>[6x]MSGPKKYFPIPVEHLEEEIRIRSADDCKQFREEFNSLPSGHIQGTFELANKEENREKNRYPNILPNDHSRVILSQLDGIPCSDYINASYIDGYKEKNKFIAAQGPKQETVNDFWRMVWEQKSATIVMLTNLKERKEEKCHQYWPDQGCWTYGNIRVCVEDCVVLVDYTIRKFCIQPQLPDGCKAPRLVSQLHFTSWPDFGVPFTPIGMLKFLKKVKTLNPVHAGPIVVHCSAGVGRTGTFIVIDAMMAMMHAEQKVDVFEFVSRIRNQRPQMVQTDMQYTFIYQALLEYYLYGDTELDVSSLEKHLQTMHGTTTHFDKIGLEEEFRKLTNVRIMKENMRTGNLPANMKKARVIQIIPYDFNRVILSMKRGQEYTDYINASFIDGYRQKDYFIATQGPLAHTVEDFWRMIWEWKSHTIVMLTEVQEREQDKCYQYWPTEGSVTHGEITIEIKNDTLSEAISIRDFLVTLNQPQARQGEQVRVVRQFHFHGWPEIGIPAEGKGMIDLIAAVQKQQQQTGNHPITVHCSAGAGRTGTFIALSNILERVKAEGLLDVFQAVKSLRLQRPHMVQTLEQYEFCYKVVQDFIDIFSDYAAHHHHHH

Protein tyrosine phosphatases (PTPs) play a critical role in regulating cellular functions by selectively dephosphorylating their substrates. The ∼280 residue PTP catalytic domain consists of an α/β structure, and biochemical and structural studies have led to a detailed understanding of the catalytic mechanism (Barford et al., 1994; Zhang, 2002). Key features of the domain include the PTP signature motif, the mobile Trp-Pro-Asp “WPD” loop that in the closed conformation positions the conserved and catalytically important aspartate residue, and the phosphotyrosine recognition loop. Here we report the crystal structures of 22 PTP domains, including two tandem-domain RPTP structures and a detailed structural comparison of this protein family.

We also report here structures of two tandem-domain RPTPs, RPTPɛ and RPTPγ, revealing the domain organization for the PTP subgroups R4 and R5. Superimposition of all five tandem-domain RPTP structures (CD45, LAR, RPTPσ, RPTPγ, and RPTPɛ) showed that the orientation of the D1 and D2 domains is highly conserved and root mean square deviation (rmsd) values of less than 4.4 Å were obtained, for each pairwise comparison, considering Cα positions of both domains. Surprisingly, sedimentation velocity measurements showed that all single-domain RPTPs studied (IA2, IA2β, GLEPP1, DEP1, and STEP) were entirely monomeric in solution, as were tandem-domain receptor PTPs (RPTPα, CD45, RPTPɛ, and RPTPμ). The determined molecular masses calculated from AUC velocity data ranged from 68.5 kDa to 74.2 kDa in agreement with the theoretical mass of monomeric tandem domains. Moreover, analysis of tandem-domain structures showed that the orientation of D1 and D2 domains is highly conserved and is incompatible with the inhibitory wedge model due to a steric clash of D2 domains. In the present study we showed that this is also true for RPTPɛ, which is in the R4 subgroup together with RPTPα, the prototype of the inhibitory wedge model. In the fourth category, both the gateway and secondary pocket are blocked and the inaccessible binding cavity harbors an aromatic residue or a proline in position of Arg24. The second-site loop assumes a twisted conformation in these phosphatases. This architecture is present in the subgroups NT5 (PTPH1, MEG1), NT6 (PTPD1, PTPD2), R1 (CD45), R2B (RPTPμ, RPTPκ, RPTPρ), and R4 (RPTPα, RPTPɛ). RPTPα, RPTPɛ, and RPTPσ displayed a more limited peptide recognition capacity in vitro, which may be related to the presence of a bulky residue in the gateway region.> GPAKEIPEVLVDPRSRRRYVRGRF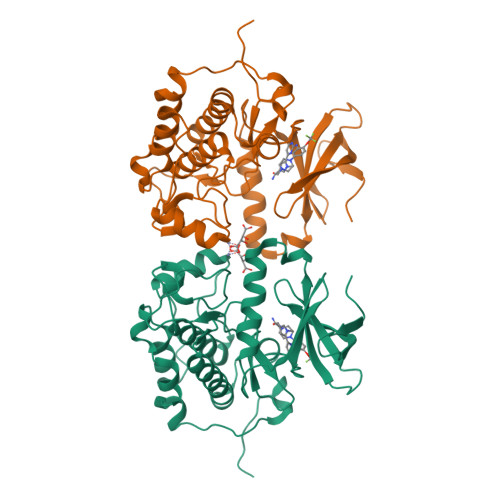LGKGGFAKCFEISDADTKEVFAGKIVPKSLLLKPHQREKMSMEISIHRSLAHQHVVGFHGFFEDNDFVFVVLELCRRRSLLELHKRRKALTEPEARYYLRQIVLGCQYLHRNRVIHRDLKLGNLFLNEDLEVKIGDFGLATKVEYDGERKKTLCGTPNYIAPEVLSKKGHSFEVDVWSIGCIMYTLLVGKPPFETSCLKETYLRIKKNEYSIPKHINPVAASLIQKMLQTDPTARPTINELLNDEFFTSGYIPARLPITCLTIPPRFSIAPSSLDPSNRKPLTVLNK> VSDAAERNLAFALSELDRITAQLKLPRHVEEEAARLYREAVRKGLIRGRSIESVMAACVYAACRLLKVPRTLDEIADIARVDKKEIGRSYRFIARNLNLTPKKLFVKPTDYVNKFA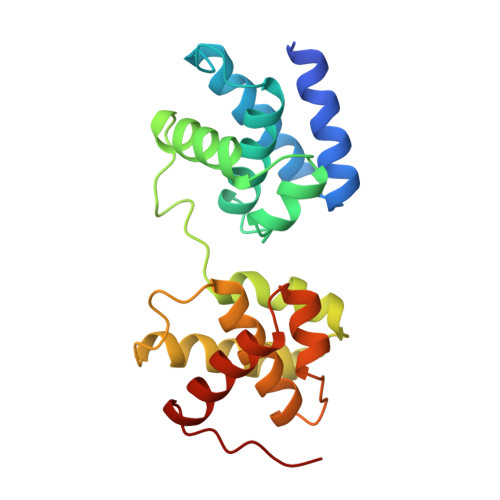DELGLSEKVRRRAIEILDEAYKRGLTSGKSPAGLVAAALYIASLLEGEKRTQREVAEVARVTEVTVRNRYKELVEKLKIKVPIA> MYAYNGKLLDVDLTREKVKEVELSEDVLKKFYGGRGLGTYILWKELG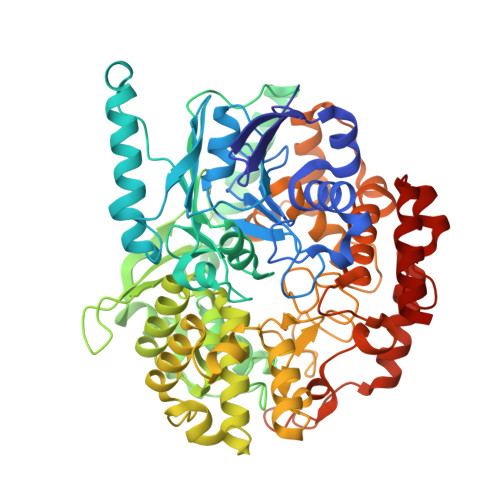EKWEKVDPLGEENLLLILTGPLTGYYPGMKTSIVSKSPESNGVVGSVLSSELGLELKAAGYDGIIIRGKAKSPVYLFIHNDTVEIRDATKYWGMGGIELYKTLLKEVHEEIRKKEKLKGVPKEPAMIYIGKGGENKVRFAAIMTKLMHAAGYGGYGAVMGSKNLKAVIAKGSGPLPEVYDKEKMKVLLREFWKELFSMTTFREWGTGAGGYSVGHDRSSEPIRNWQEEYHDNEEISVVNFENRTWIKKYWADYGCPVNCMKISYLRYGPYKGSISDAPDYELQAYMGTNLGIFEPEKIVYLSYLVDELGLDGINTGNILGFAAELYQRGILTKEDLGFELNWGDEKAFAKLLHLIVEKEGIGKILAEGTYRAALKISEIKGIDVTKYAVHVKGIAVGAHGIRSELDYTKDISYAVSVQGGDHTSTAALPAKGYTGELVEAFYDSAVICNFVTKPGFEKIIEFGNALSGFNITPEQWLNEIGLRIIHLQRILLLLGGPDVYWDPRKDDDNPPRFYEPLPSGPVKGKAPNREDIKAKVKQYYEEIGYDEHGIPKEEVLEELGIGEAKREVKRIKKRLN N-[(1R)-1-(2-chlorophenyl)ethyl]methanesulfonamide 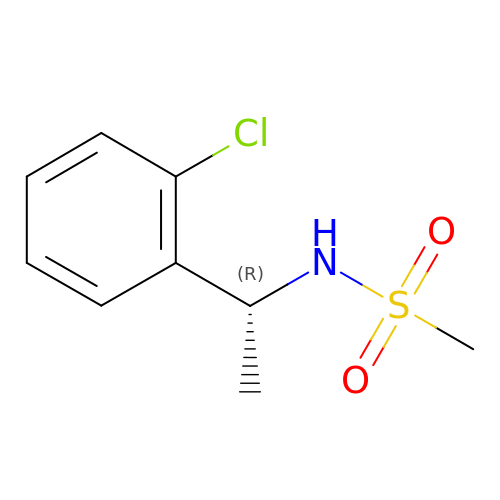| C9 H12 Cl N O2 S | HMJIOKFBRSKMHO-SSDOTTSWSA-N>[4x]CTAITYVSKDHYFGRNFDYEISYNEVVTITPRNYKFSFREVGNLDHHFAIIGIAAGIADYPLYYDAINEKGLGMA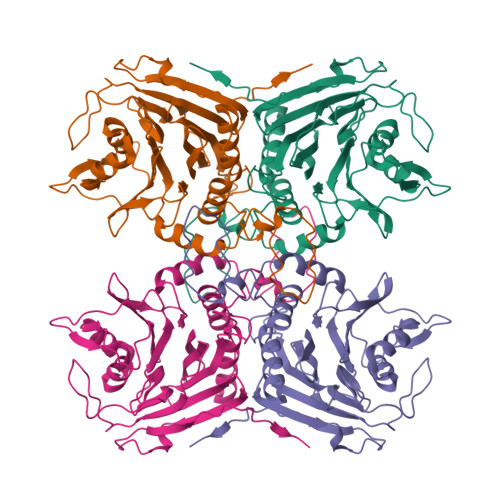GLNFSGYADYKKIEEGKENVSPFEFIPWVLGQCSTVDEAKKLLKNLNLVNINFSDELPLSPLHWLLADKEQSIVVESTKEGLRVFDNPVGVLTNNPTFDYQLFNLNNYRVLSTRTPKNNFSDQIELDIYSRGMGGIGLPGDLSSVSRFVKATFTKLNSVSRSSEYESISQFFHILSSVEQQKGLCDVGDEKYAYTIYSSCCNLEKGIYYYRTYDNSQITAVDMNKENLEKDSLIVYPMVETQQINYANHHHHHH V-ATPases function as proton pumps in acidic organelles and plasma membranes of eukaryotic cells. Furthermore, E. hirae V-ATPase physiologically functions as an ion pump, similar to eukaryotic V-ATPases34353637, and is composed of nine subunits with amino acid sequences that are homologous to those of the corresponding subunits of eukaryotic V-ATPases638. Thus, the V1 motor achieves its rotational dynamics via several conformational changes that are generated by the binding of ATP, release of Pi and ADP, and cooperative coupling among these conformational changes.

Next, we soaked the crystals of eV1 in 20 μM ADP, and the crystal structure (denoted 2ADPV1) was solved at a resolution of 3.3 Å. Two ADP:Mg2+ molecules were bound to the ‘bound' and ‘tight' forms of eV1, as in the case of 2ATPV1, and induced conformational changes with the crystal packing rearrangements. The eV1 ‘bound' form did not show a conformational change upon ADP binding (r.m.s.d.=0.48 Å). However, the eV1 ‘tight' form changed to a more open conformation (AC from ACR; BC' from BCR) upon ADP binding. We designated the new ADP-bound ACBC' pair of 2ADPV1 as the ‘ADP-bound' form. According to the observed conformational changes, the DF axis became tilted towards the ‘ADP-bound' form to maintain the extensive protein–protein interactions between DF and the ‘ADP-bound' form. The last conformation of the AB pair (eV1-‘empty'), which did not bind to ADP, also showed a cooperative conformational change. Specifically, Eh-A (AO) and Eh-B (BC) of the ‘empty' form were attracted to the DF axis and the ‘ADP-bound' form, respectively. The wider conformation of the resultant AB (AO'BO'') pair was most similar to that of the eA3B3-‘bindable' form (AO'BO: ATP-accessible state) among all AB pairs (r.m.s.d.=0.94 Å), and was thus denoted a ‘bindable-like' form. Based on these findings, we inferred that the structure of 2ADPV1 corresponds to the state of waiting for ATP binding (that is, the ATP-binding dwell) in the rotation.

>[3x]GSSGSSGMQIGKIIKVSGPLVMAENMSEASIQDMCLVGDLGVIGEIIEMRQDVASIQVYEETSGIGPGEPVRSTGEALSVELGPGIISQMFDGIQRPLDTFMEVTQSNFLGRGVQLPALDHEKQWWFEATIEEGTEVSAGDIIGYVDETKIIQHKIMVPNGIKGTVQKIESGSFTIDDPICVIETEQGLKELTMMQKWPVRRGRPIKQKLNPDVPMITGQRVIDTFFPVTKGGAAAVPGPFGAGKTVVQHQIAKWSDVDLVVYVGCGERGNEMTDVVNEFPELIDPNTGESLMERTVLIANTSNMPVAAREASIYTGITIAEYFRDMGYDVAIMADSTSRWAEALREMSGRLEEMPGDEGYPAYLGSRLAEYYERSGRVIALGSDQREGSITAISAVSPSGGDISEPVTQNTLRVVKVFWGLDSSLAQKRHFPSINWIQSYSLYSTEVGRYMDQILQQDWSDMVTEGMRILQEEEQLNEIVRLVGIDSLSDNDRLTLEVAKSIREDYLQQNAFDDVDTFTSREKQFNMLKVILTFGKEARKALSLGAYFNEIMEGTVAVRERISRSKYIPEEELAKISSINEEIKETIQLIVSEGGMTDD;>[3x]GSSGSSGMIKEYRTIKEVVGPLMAVEKVSGVKYEELIEVRMQNGEIRRGQVLEVQEDKAMVQIFEGTSGINLKNSSVRFLGHPLQLGVSEDMIGRVFDGLGRPKDNGPEILPEKYLDINGEVINPIARDYPDEFIQTGISAIDHLNTLVRGQKLPVFSGSGLPHKELAAQIARQATVLDSSDDFAVVFAAIGITFEEAEFFMEDFRQTGAIDRSVMFMNLANDPAIERIATPRMALTAAEYLAYEKGMHVLVIMTDMTNYAEALREISAARREVPGRRGYPGYLYTNLATLFERAGRIRGLKGSVTQIPILTMPEDDKTHPIPDLTGYITEGQIILTRELYKSGIQPPIDVLPSLSRLKDKGTGAGKTREDHAATMNQLFAAYAQGKQAKELAVVLGESALSDIDKIYAKFAERFENEYVNQGFYTNRTITETLDLGWELLAMLPRTELKRIKDDLLDKYLPEGK;> GSSGSSGMRLNVNPTRMELTRLKKQLTTATRGHKLLKDKQDELMRQFILLIRKNNELRQAIEKETQTAMKDFVLAKSTVEEAFIDELLALPAENVSISVVEKNIMSVKVPLMNFQYDETLNETPLEYGYLHSNAELDRSIDGFTQLLPKLLKLAEVEKTCQLMAEEIEKTRRRVNALEYMTIPQLEETIYYIKMKLEENERAEVTRLIKVKNMGTEE;> MTYKIGVVGDKDSVSPFRLFGFDVQHGTTKTEIRKTIDEMAKNEYGVIYITEQCANLVPETIERYKGQLTPAIILIPSHQGTLGIGLEEIQNSVEKAVGQNILSGPSSGENLYFQ>[2x]MTGMSREEVESLIQEVLEVYPEKARKDRNKHLAVNDPAVTQSKKCIISNKKSQPGLMTIRGCAYAGSKGVVWGPIKDMIHISHGPVGCGQYSRAGRRNYYIGTTGVNAFVTMNFTSDFQEKDIVFGGDKKLAKLIDEVETLFPLNKGISVQSECPIGLIGDDIESVSKVKGAELSKTIVPVRCEGFRGVSQSLGQHIANDAVRDWVLGKRDEDTTFASTPYDVAIIGDYNIGGDAWSSRILLEEMGLRCVAQWSGDGSISEIELTPKVKLNLVHCYRSMNYISRHMEEKYGIPWMEYNFFGPTKTIESLRAIAAKFDESIQKKCEEVIAKYKPEWEAVVAKYRPRLEGKRVMLYIGGLRPRHVIGAYEDLGMEVVGTGYEFAHNDDYDRTMKEMGDSTLLYDDVTGYEFEEFVKRIKPDLIGSGIKEKFIFQKMGIPFREMHSWDYSGPYHGFDGFAIFARDMDMTLNNPCWKKLQAPWEASEGAEKVAASA;>MSQQVDKIKASYPLFLDQDYKDMLAKKRDGFEEKYPQDKIDEVFQWTTTKEYQELNFQREALTVNPAKACQPLGAVLCALGFEKTMPYVHGSQGCVAYFRSYFNRHFREPVSCVSDSMTEDAAVFGGQQNM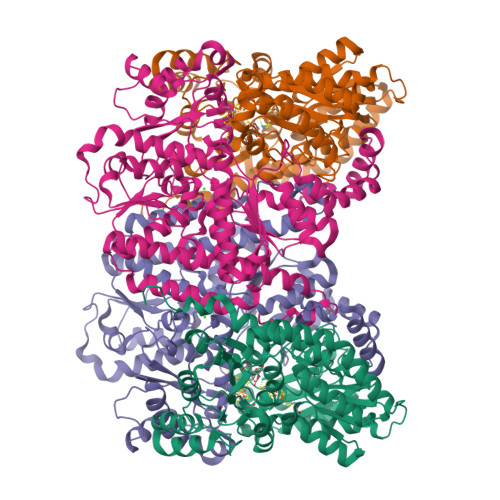KDGLQNCKATYKPDMIAVSTTCMAEVIGDDLNAFINNSKKEGFIPDEFPVPFAHTPSFVGSHVTGWDNMFEGIARYFTLKSMDDKVVGSNKKINIVPGFETYLGNFRVIKRMLSEMGVGYSLLSDPEEVLDTPADGQFRMYAGGTTQEEMKDAPNALNTVLLQPWHLEKTKKFVEGTWKHEVPKLNIPMGLDWTDEFLMKVSEISGQPIPASLTKERGRLVDMMTDSHTWLHGKRFALWGDPDFVMGLVKFLLELGCEPVHILCHNGNKRWKKAVDAILAASPYGKNATVYIGKDLWHLRSLVFTDKPDFMIGNSYGKFIQRDTLHKGKEFEVPLIRIGFPIFDRHHLHRSTTLGYEGAMQILTTLVNSILERLDEETRGMQATDYNHDLVR[2x]>[4x]MRGSHHHHHHGSMKRAVITGLGIVSSI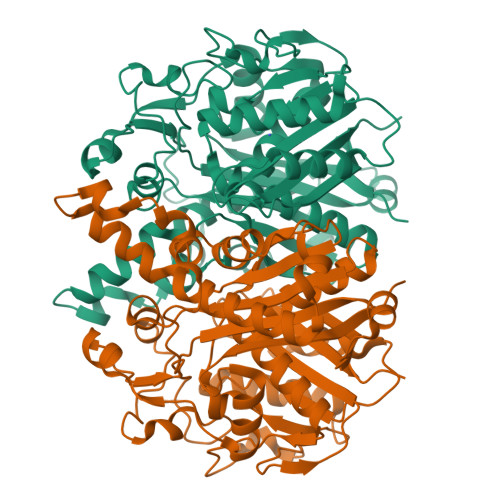GNNQQEVLASLREGRSGITFSQELKDSGMRSHVWGNVKLDTTGLIDRKVVRFMSDASIYAFLSMEQAIADAGLSPEAYQNNPRVGLIAGSGGGSPRFQVFGADAMRGPRGLKAVGPYVVTKAMASGVSACLATPFKIHGVNYSISSACATSAHCIGNAVEQIQLGKQDIVFAGGGEELCWEMACEFDAMGALSTKYNDTPEKASRTYDAHRDGFVIAGGGGMVVVEELEHALARGAHIYAEIVGYGATSDGADMVAPSGEGAVRCMKMAMHGVDTPIDYLNSEGTSTPVGDVKELAAIREVFGDKSPAISATKAMTGHSLGAAGVQEAIYSLLMLEHGFIAPSINIEELDEQAAGLNIVTETTDRELTTVMSNSFGFGGTNATLVMRKLKD>HHHHHHGSMAEKDDTAQVVVNNNDPTYKSEHTDTLVYNPEGALSYRLIAQHVEYYSDQAVSWFTQPVLTTFDKDKIPTWSVKADKAKLTNDRMLYLYGHVEVNALVPDSQLRRITTDNAQINLVTQDVTSEDLVTLYRTTFNSSGLKMRGNLRSKNAELIEKVRTSYEIQNKQTQP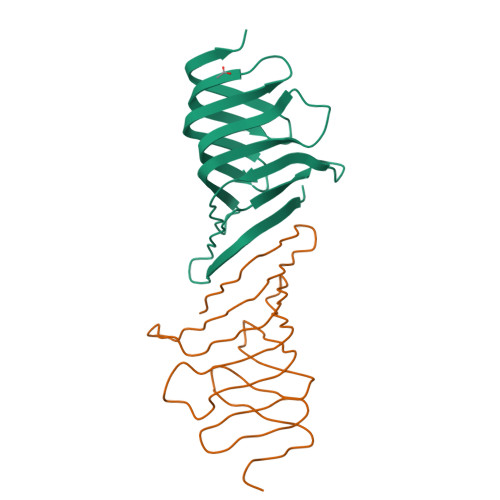[2x]>HHHHHHSSGLVPRGSHMETGTKTYEGAKAYKRSPHGELFTLVASSLFLGDNTYYEYGGERVERFINLATTLSKEDPEYVASLANYARNELGLRSNPAALVAHLFYSNALEERRDLILATTKKVWQRGDDHLETLAYVKAVGWKLRSALKKAIAERLNDIPPSLLLKYKRARRVVSQRLAIRLTHPRPRDEERSLLFQYIVKGSRASEEAKKLAEEVMEERPTWERIISSKGSTPETWLEALPHLNGLSLVRNLNNLFKHGLLENLEVK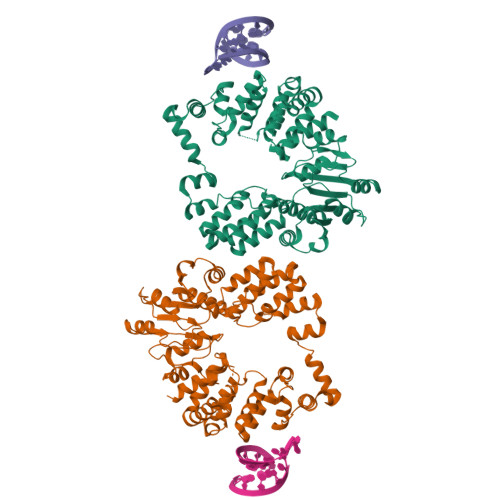KTIEDKFSRSGSWKIFPFQYYSALKMGEKEGWPYWIMALLEEALESSAPETRLEGETLFLVDVSGSMYYPVSRNSNLHMAEAASVLATVLVKRLGGELWTFADEAQDYTGHTHLSTYSLVRKIVREGRGGTYLERAIRKAILDRSWTGRRVVIITDEQTHDMPWEALKDWLRSGENRVAHIINVAGYLPTAFPEDRIAKVGGWSDKIITLIESLEVGEEGIRNFLVSNYLPP[2x]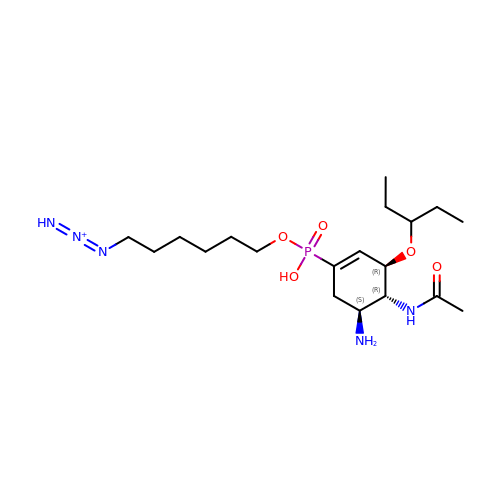6-[[(3~{R},4~{R},5~{S})-4-acetamido-5-azanyl-3-pentan-3-yloxy-cyclohexen-1-yl]-oxidanyl-phosphoryl]oxyhexylimino-azanylidene-azanium | C19 H37 N5 O5 P | SQYBSQHYIJSZEH-IPMKNSEASA-O>[3x]MRIVQPVIEQLKAQSHPVCHYIYDLVGLEHHLQHITSSLPSNCQMYYAMKANSERTILDTISQYVEGFEVASQGEIAKGLAFKPANHIIFGGPGKTDEELRYAVSEGVQRIHVESMH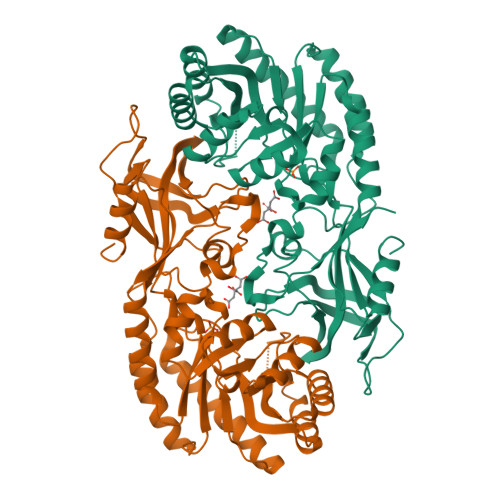ELQRLNAILEDEDKTQHILLRVNLAGPFPNATLHMAGRPTQFGISEDEVDDVIEAALVMPNIHLDGFHFHSISNNLDSNLHVDVVKLYFKKAKSWSEKHRFPLKHINLGGGIGVNYADLTSQFEWDNFVENFKTLIVEQEMEDVTLNFECGRFIVAHIGYYVTEVLDIKKVHGAWYAILRGGTQQFRLPVSWQHNHPFEIYRYKDNPYSFEKVSISRQDTTLVGQLCTPKDVFAREVQIDAISTGDVIVFKYAGAYGWSISHHDFLSHPHPEFIYLTQTKEDEHHHHHH>[6x]MGSDKIHHHHHHENLYFQGMNETPLRLLEMLTQTREDLWRAAQALTERGVTRIILTGSGTSYHGALT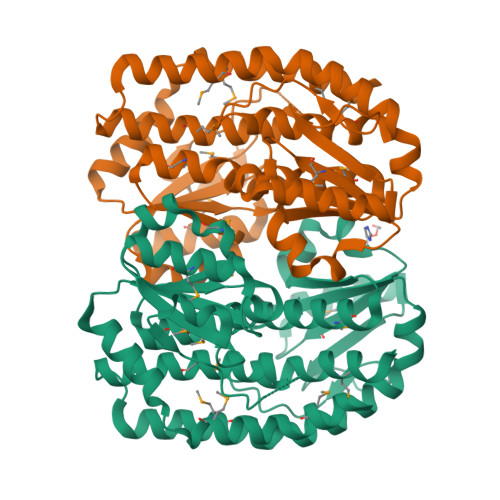ARTFMQRWCALPVDVCWPFMLDDETLARSGKALVVGISQGGGSLSTLAAMERARNVGHITASMAGVAPATIDRAADYILTVPCGEETAGAKTKGYHCTVLNLMLLALAVAGQQQRLDGEQRRSLLLRMEKTFNHLPALVTASQAWAQTNALALRDSADIRLTGPATLFGTVQEGALKMLETLRCPVSGYEFEEFIHGIYNAFNAQSALIMLDPQPDARQDRLAQILGEWTPSIYRIGPQVENNGLNLNFPFVNDEDFAVFEYIIPLQMLCAILPPQKGINPAIPKDPQFHQKMKSKQEI NOD1 and NOD2 (Nucleotide-binding oligomerization domain-containing proteins 1 and 2) are cytosolic receptors of the innate immune system, which respond to intracellular fragments of the bacterial peptidoglycans, D-glutamyl-meso-diaminopimelic acid (iE-DAP) and muramyl dipeptide (MPD), respectively. Upon ligand recognition, NOD receptors oligomerise and recruit an adaptor protein, Receptor Interacting protein kinase 2 (RIP2), through interactions of their respective CARD domains. RIP2 also contains an N-terminal dual-specificity ser/tyr kinase domain (RIP2K), which belongs to the TKL kinase family (Tyrosine kinase-like). RIP2 undergoes auto-phosphorylation and K-63 linked ubiquitination at Lys209, becoming a scaffolding protein for downstream effectors.

As expected from the phosphorylation profile, RIP2K-AMPPCP show a typical active state, within AMPPCP bound the active state between the N-and C-lobes. All essential functional elements are in their canonical positions. The R-spine is aligned, the DFG motif is in the expected IN conformation, the Helix αC is inwardly displaced and Glu66 in Helix αC (Glu91 in PKA) forms a salt bridge with Lys47 from strand β3 (Lys 72 in PKA). Only residues 164–172 and 186–196 could be traced for RIP2K-AMPPCP chain B, implying that there is no electron density for any of the phosphorylation sites detected by mass spectrometry. The AS is close to the loop containing the site of ubiquitination Lys209 (residues 200–210, referred to here as the Lys209 loop), which is also disordered. Both structures crystallised in the tetragonal space group P41212 with a dimer in the asymmetric unit, in agreement with the size exclusion chromatography profile. Within the dimer interface, the 2-fold symmetry related N-termini (residues 6–9) form anti-parallel β-strands. In the RIP2K-AMPPCP structure, there is an extensive hydrogen-bonding (H-bond) network linking together Helix αC and the ordered part of the AS with their surroundings including the N-terminal anti-parallel β-strands. Therefore, the active conformation of RIP2K is stabilised by a specific H-bond network which connects Helix αC with the magnesium binding loop, the AS, and the N-terminus without involving any phosphorylation site. In the active conformation, the 2-fold symmetry related N-termini (residues 6–9) form anti-parallel β-strands that are further stabilized by His71 from Helix αC and Arg74. The active state of RIP2K is phosphorylated at the AS and is a compact dimer both in solution and in crystals, as seen in this work and other recent publications, where an extra helix (Helix αJ) at the C-terminus of the kinase domain has been observed to reinforce the dimerization interface.

>[2x]GAMAMNGEAICSALPTIPYHKLADLRYLSRGASGTVSSARHADWRVQVAVKHLHIHTPLLDSERKDVLREAEILHKARFSYILPILGICNEPEFLGIVTEYMPNGSLNELLHRKTEYPDVAWPLRFRILHEIALGVNYLHNMTPPLLHHDLKTQNILLDNEFHVKIADFGLSKWRMMSLSQSRSSKSAPEGGTIIYMPPENYEPGQKSRASIKHDIYSYAVITWEVLSRKQPFEDVTNPLQIMYSVSQGHRPVINEESLPYDIPHRARMISLIESGWAQNPDERPSFLKCLIELEPVFRTFEEI> GPAAGAVATGEYRNLFAEIGKSEIDIQRKIDEAFQHLFYGDAKDAAVYYQAGGNENGPLAYVYDVNSNDVRSEGMSYGMMITVQMDKKAEFDAIWNWAKTYMYQDSPTHPAFGYFAWSMRRDGVANDDMPAPDGEEYFVTALYFAAARWGNGEGIFNYQQEADTILSRMRHRQVITGPTNRGVMTATNLFHPEEAQVRFTPDINNADHTDASYHLPSFYEIWARVAPQEDRAFWAKAADVSRDYFAKAAHPVTALTPDYGNFDGTPWAASWRPESVDFRYDAWRSVMNWSMDYAWWGKDSGAPARSDKLLAFFETQEGKMNHLYSLDGKPLGGGPTLGLISMNATAAMAATDPRWHNFVEKLWQQQPPTGQYRYYDGVLYLMA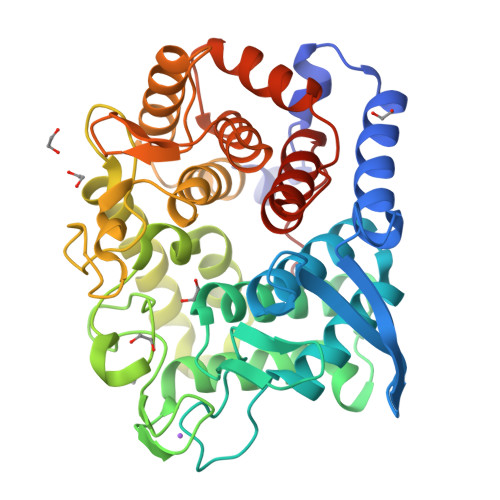LLHCAGEYKAWIPDGE(7P,8S)-7-[(2S)-2-methyl-2,3-dihydro-1-benzofuran-5-yl][1,2,4]triazolo[1,5-a]pyrimidine | C14 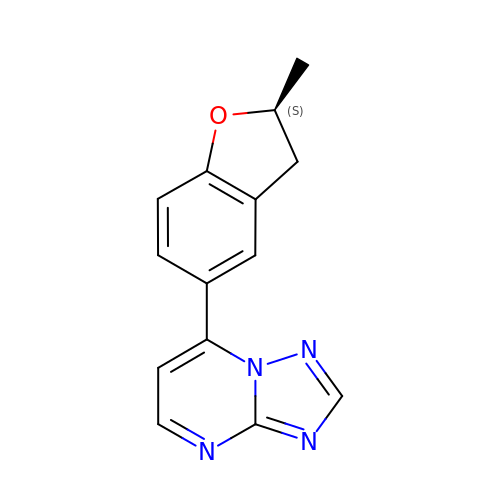H12 N4 O | BPKWKBIVZRWWQO-VIFPVBQESA-N> GPLGSMDSSQLHVAIVSSPGMGHLIPVLVLGNRLATHHNIKITILAITTTSSSAETEFLKKTTLTNEEKTIEIIPVPSVDISHLINSSTKIFTQLRLLVREALPKIHSTIASMTHRPDALIVDIFCTQILPIAEEFNISKYTYHPTTAWTLALAIYCQVFDKEIEGEYVELKEPLKIPGCKALRPDDVVDPLLDRSDQQYEEYVKLGKEYTDFDGILINTWEDLEPETINALRYNEKLRLLLKVPVFPIGPLRRKVETTLNDEVIQWLDKQNNESVLFVSFGSGGTLSTKQMTELAWGLEL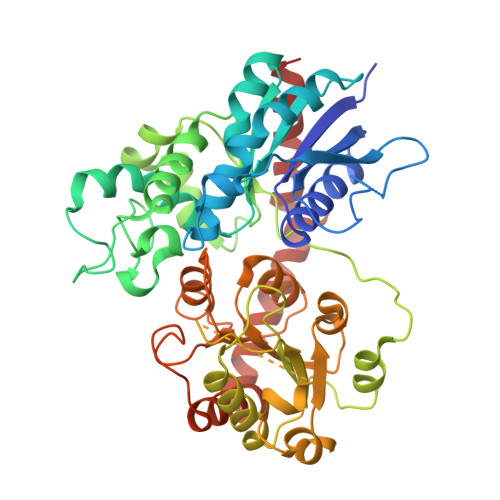SQQKFVWVVRPPSDGDADSAYLNSAGKDTRDMSEYLPEGFLTRTKDMGLVVPMWANQVEILSHSSVGGFLTHCGWNSTVESLTNGVPMIAWPLHAEQKMNAAMLTEELGVAIRPAVLPTKKLVKREEIQGMVRILMQTKEGKRIKEKAKKLKKSAENALSDGGSSYNSICELVKDIRSREL> GGLEKDFLPLYFGWFLTKKSSETLRKAGQVFLEELGNHKAFKKELRHFISGDEPKEKLELVSYFGKRPPGVLQCTTKFCDYGKAAGAEEYAQQEVVKRSYGKAFKLSISALFVTPKTAGAQVVLTDQELQLWPSDLDKPSASEGLPPGSRAHVTLGCAADVQPVQTGLDLLDILQQVKGGSQGEAVGELPRGKLYSLGKGRWMLSLTKKMEVKAIFTGYYG

2′,3′-cyclic nucleotide 3′-phosphodiesterase (CNPase) comprises 4% of total myelin protein in the central nervous system (CNS), being the most abundant CNS non-compact myelin protein4. CNPase consists of an N-terminal polynucleotide kinase-like domain10, a catalytic phosphodiesterase domain11, and a membrane-anchored C-terminal tail, which contains a cysteine residue that undergoes isoprenylation. The catalytic domain enables the rapid hydrolysis of nucleoside 2′,3′-cyclic phosphates to nucleoside 2′-phosphates. The CNPase catalytic site, lying in a groove between two lobes, has pseudo two-fold symmetry and contains two apposing His-X-Thr-X (X denotes a hydrophobic residue) motifs, characteristic for 2H phosphoesterases 113537.

In mouse CNPase, this is done by His230, Thr232, His309, and Thr311, in a manner, where a nucleophilic water molecule activated by His309 can attack the cyclic phosphate and a pentavalent transition state is formed. Mutation of active-site histidine residues (H230Q, H230S, H309Q, H309S, and H230Q/H309Q double mutant) abolishes CNPase activity. Overall, the structures of H230S, H309S, H230Q, H309Q, and H230Q/H309Q are highly similar.>[2x]GAMALPSGSDPAFSQPKSVLDAGLTCQGASPSSVSKPILLVPGTGTTGPQSFDSNWIPLSAQLGYTPCWISPPPFMLNDTQVNTEYMVNAITTLYAGSGNNKLPVLTWSQGGLVAQWGLTFFPSIRSKVDRLMAFAPDYKGTVLAGPLDALAVSAPSVWQQTTGSALTTALRNAGGLTQIVPTTNLYSATDEICQPQVSNSPLDSSYLFNGKNVQAQAVCGPLFVIDHAGSL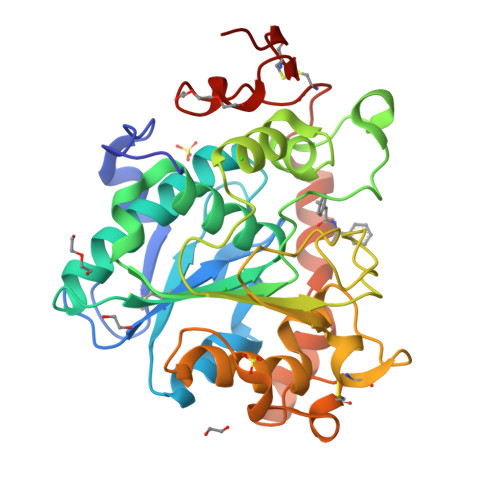TSQFSYVVGRSALRSTTGQARSADYGITDCNPLPANDLTPEQKVAAAALLAPGVAAIVAGPKQNCEPDLMPYARPFAVGKRTCSGIVTP>MDLAKLGLKEVMPTKINLEGLVGDHAFSMEGVGEGNILEGTQEVKISVTKGAPLPFAFDIVSVAFTYGNRAYTGYPEEISDYFLQSFPEGFTYERNIRYQDGGTAIVKSDISLEDGKFIVNVDFKAKDLRRMGPVMQQDIVGMQPSYESMYTNVTSVIGECIIAFKLQTGKHFTYHMRTVYKSKKPVETMPLYHFIQHRLVKTNVDTASGYVVQHETAIAAHSTIKKIEGSLP[6x];>[6x]MTSKVYDPEQRKRMITGPQWWARCKQMNVLDSFINYYDSEKHAENAVIFLHGNATSSYLWRHVVPHIEPVARCIIPDLIGMGKSGKSGNGSYRLLDHYKYLTAWFELLNLPKKIIFVGHDWGAALAFHYAYEHQDRIKAIVHMESVVDVIESWDEWP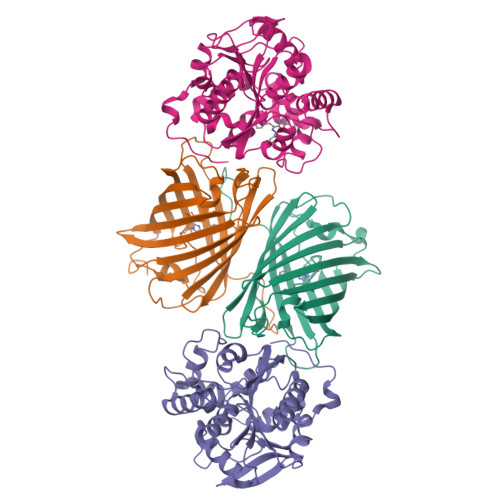DIEEDIALIKSEEGEKMVLENNFFVETVLPSKIMRKLEPEEFAAYLEPFKEKGEVRRPTLSWPREIPLVKGGKPDVVQIVRNYNAYLRASDDLPKLFIESDPGFFSNAIVEGAKKFPNTEFVKVKGLHFLQEDAPDEMGKYIKSFVERVLKNEQSGLEVLFQ>REEEDVICDGCNGPVVGTRYKCSVCPDYDLCSVCEGKGLHRGHTKLAFPSPFGHLSEGFS[2x]

Intriguingly, the autophagy adapter p62/SQSTM1/Sequestosome-1 was recently reported to recognize N-degrons, the N-end rule substrates of the well-characterized UPS, and where ultimately these substrates are delivered to ALS8,9. p62 is a key selective autophagy adapter that plays a role in the degradation of various cellular constituents such as misfolded proteins and their aggregates, malfunctioning organelles, and invading pathogens. Intriguingly, it was recently reported that the central ZZ-domain in p62 plays a critical role in the recognition of N-terminal arginylated BiP/GRP78 by the Arg-tRNA transferase ATE1. Here, we present the high resolution structures of the ZZ-domain of p62 in complex with 8 different N-degrons including type-1 and type-2, and subsequently identify key determinants involved in the unusual recognition.

In an effort to elucidate the manner by which the ZZ-domain of p62 recognizes N-terminal arginylated BiP/GRP78 (hereafter referred to as R-BiP), we generated the chimeric protein N-terminal R-BiP (R*-E19b-E20b-E21b-D22b; where “*” and subscript “b” represent attachment to the modified N-terminus and BiP residues, respectively) fused to the ZZ-domain using a special expression system. Using this fusion protein, we determined the complex structure of the ZZ-domain with R-BiP substrate at 1.45 Å resolution. As expected, the binding site of the ZZ-domain comprises a negatively charged patch for recognition of the positively charged N-terminal NH3+ group of R-BiP. The side chains of Asp129 and Asp149 in the ZZ-domain form hydrogen bonds with the α-amino group of R-BiP. Moreover, the key carboxylate of Asp129 which is involved in recognizing the α-amino group also forms an ionic interaction with the guanidinium group of the N-terminal arginine residue. Another negatively charged residue, Asp147, also participates in the N-degron binding, and in a manner that is not sequence-specific. The side chain carboxylate of Asp147 interacts with the main chain nitrogen atom of the first peptide bond between the first arginine R* and Glu19b of the N-degron. The main chain nitrogen atom of Ile127 also forms a hydrogen bond with the carbonyl oxygen of the first peptide bond of the N-degron. However, the side chain of Asn132 is re-oriented to form a specific interaction with the side chain of the N-degron. It is rotated 72.3° and moved by approximately 3.0 Å to facilitate recognition of the guanidinium group of the N-terminal arginine.>MENGSGKVLKPMDSEQLREYGHLMVDFIADYYKTIEDFPVLSQVQPGYLHKLLPDSAPDHPETLDQVLDDVRAKILPGVTHWQSPSFFAYYPSNSSVAGFLGEMLSAGLGIVGFSWVTSPAATELEMIVLDWVAKLLNLPEQFMSKGNGGGVIQGSASEAVLVVLIAARDKVLRSVGKNALEKLVVYSSDQTHSALQKACQIAGIHPENCRVLTTDSSTNYALRPESLQEAVSRDLEAGLIPFFLCANVGTTSSTAVDPLAALGKIANSNGIWFHVDAAYAGSACICPEYRQYIDGVETADSFNMNAHKWFLTNFDCSLLWVKDQDSLTLALSTNPEFLKNKASQANLVVDYKDWQIPLGRRFRSLKLWMVLRLYGSETLKSYIRNHIKLAKEFEQLVSQDPNFEIVTPRIFALVCFRLVPVKDEEKKCN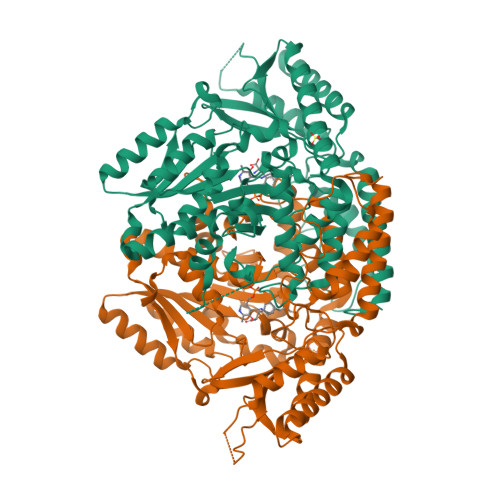NRNRELLDAVNSSGKLFMSHTALSGKIVLRCAIGAPLTEEKHVKEAWKIIQEEASYLLHK[2x]6-methoxy-1,3,4,5-tetrahydro-2H-1-benzazepin-2-one | C11 H13 N O2 | 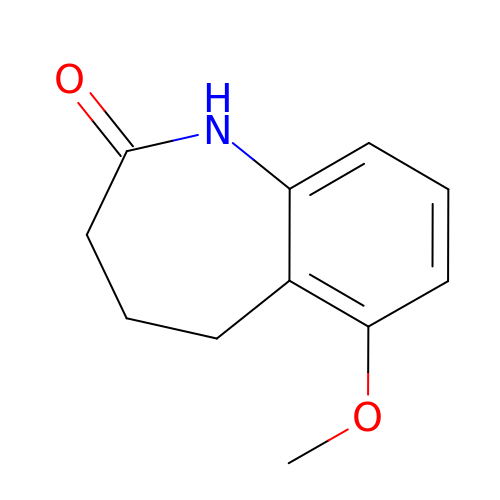NEMWEYAZCVDHEF-UHFFFAOYSA-N> PSLGKETAAAKFERQHMDSSTSAASSSNYCNQMMKSRNLTKDRCKPVNTFVHESLADVQAVCSQKNVACKNGQTNCYQSYSTMSITDCRETGSSKYPNCAYKTTQANKHIIVACEGNP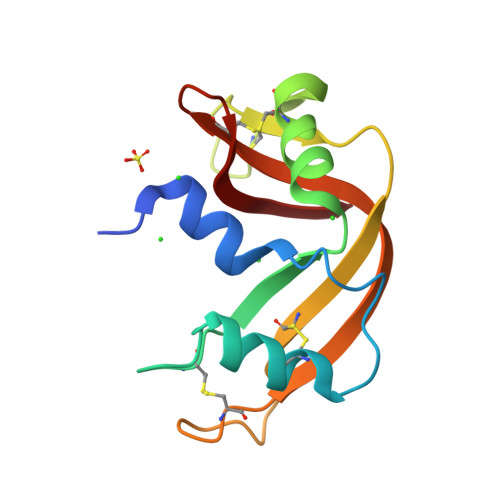YVPVHFDASV> DDVTVVYQNGLPVISVRLPSRRERCQFTLKPISDSVGVFLRQLQEEDRGIDRVAIYSPDGVRVAASTGIDLLLLDDFKLVINDLTYHVRPPKRDLLSHENAATLNDVKTLVQQLYTTLCIEQHQLNKERELIERLEDLKEQLAPLEKVRIEISRKAEKRTTLVLWGGLAYMATQFGILARLTWWEYSWDIMEPVTY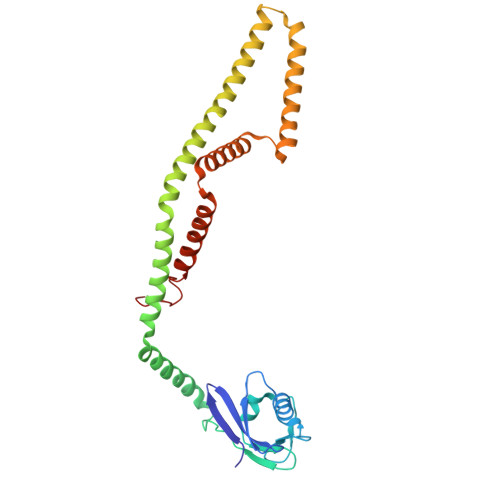FITYGSAMAMYAYFVMTRQEYVYPEARDRQYLLFFHKGAKKSRFDLEKYNQLKDAIAQAEMDLKRLRDPLQVHLPLRQIG>[2x]MTQDVTSGYSNLDLDLRDNGVCVVTLNRPDKRNALDVATIEELVTFFSTAHRKGVRAVVLTGAGDHFCAGLDLVEHWKADRSADDFMHVCLRWHEAFNKMEYGGVPIIAALRGAVVGGGLELASAAHLRVMDQSTYFALPEGQRGIFTGGGATIRVSDMIGKYRMIDMILTGRVY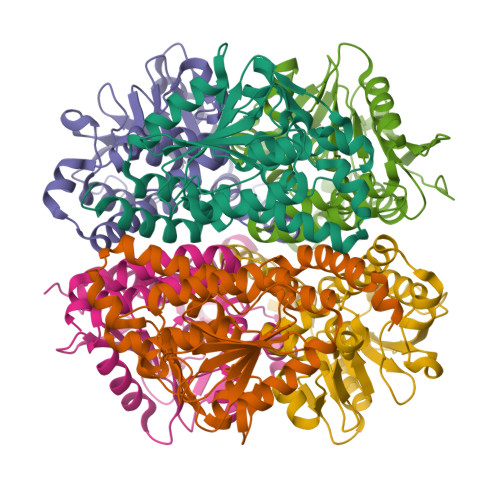QGQEAADLGLAQYITEGSSFDKAMELADKIASNLPLTNFAICSAISHMQNMSGLDAAYAEAFVGGIVNTQPAARERLEAFANKTAARVRPNSLEHHHHHH>[2x]GICKSSDCIKSAARLIQNMDATAEPCTDFFKYACGGWLKRNVIPETSSRYSNFDILRDEL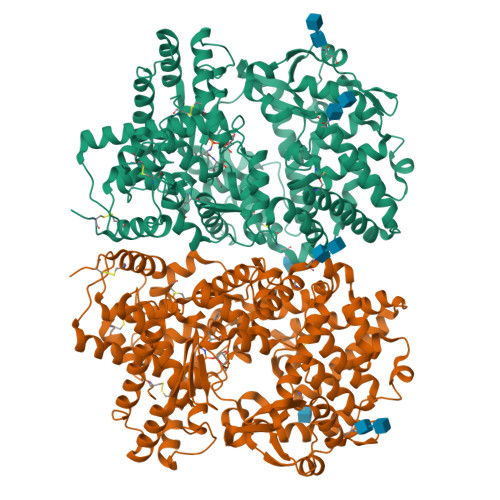EVILKDVLQEPKTEDIVAVQKAKTLYRSCVNETAIDSRGGQPLLKLLPDVYGWPVATQNWEQTYGTSWSAEKSIAQLNSKYGKKVLINFFVGTDDKNSMNHIIHIDQPRLGLPSRDYYECTGIYKEACTAYVDFMIAVAKLIRQEEGLPIDENQISVEMNKVMELEKEIANATTKSEDRNDPMLLYNKMTLAQIQNNFSLEINGKPFSWSNFTNEIMSTVNINIPNEEDVVVYAPEYLIKLKPILTKYSPRDLQNLMSWRFIMDLVSSLSRTYKDSRNAFRKALYGTTSESATWRRCANYVNGNMENAVGRLYVEAAFAGESKHVVEDLIAQIREVFIQTLDDLTWMDAETKKKAEEKALAIKERIGYPDDIVSNDNKLNNEYLELNYKEDEYFENIIQNLKFSQSKQLKKLREKVDKDEWITGAAIVNAFYSSGRNQIVFPAGILQPPFFSAQQSNSLNYGGIGMVIGHEITHGFDDNGRNFNKDGDLVDWWTQQSANNFKEQSQCMVYQYGNFSWDLAGGQHLNGINTLGENIADNGGIGQAYRAYQNYVKKNGEEKLLPGIDLNHKQLFFLNFAQVWCGTYRPEYAVNSIKTDVHSPGNFRIIGSLQNSVEFSEAFQCPKNSYMNPEKKCRVW>MEKDTKQVDIIFRSKLPDIYIPNHLPLHSYCFENISEFSSRPCLINGANKQIYTYADVELNSRKVAAGLHKQGIQPKDTIMILLPNSPEFVFAFIGASYLGAISTMANPLFTPAEVVKQAKASSAKIIVTQACHVNKVKDYAFENDVKIICIDSAPEGCLHFSVLTQANEHDIPEVEIQPDDVVALPYSSGTTGLPKGVMLTHKGLVTSVAQQVDGENPNLYIHSEDVMLCVLPLFHI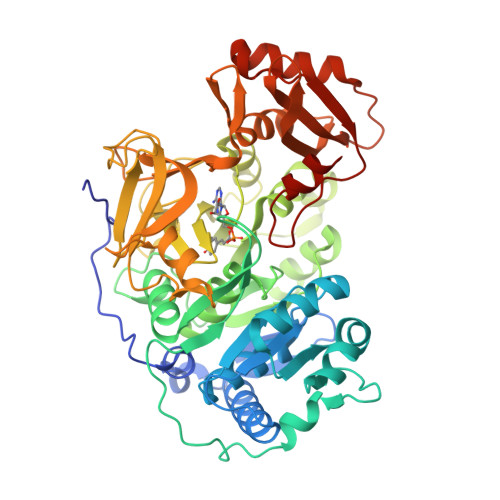YSLNSVLLCGLRVGAAILIMQKFDIVSFLELIQRYKVTIGPFVPPIVLAIAKSPMVDDYDLSSVRTVMSGAAPLGKELEDTVRAKFPNAKLGQGYGMTEAGPLAMCLAFAKEPFEIKSGACGTVVRNAEMKIVDPKTGNSLPRNQSGEICIRGDQIMKGYLNDPEATARTIDKEGWLYTGDIGYIDDDDELFIVDRLKELIKYKGFQVAPAELEALLLNHPNISDAAVVPMKDEQAGEVPVAFVVRSNGSTITEDEVKDFISKQVIFYKRIKRVFFVDAIPKSPSGKILRKDLRAKLAAGLPN[2x]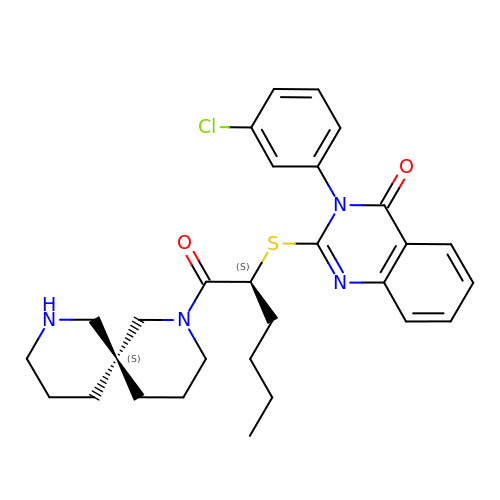3-(3-chlorophenyl)-2-({(1S)-1-[(6S)-2,8-diazaspiro[5.5]undec-2-ylcarbonyl]pentyl}sulfanyl)quinazolin-4(3H)-one | C29 H35 Cl N4 O2 S | GMBUMIBZLYNLLU-SVEHJYQDSA-N> MTDVARLLALRSFTELGARQRARALLDAGSFRELLDPFAGVQSPWLERQGIVPQADDGVVVARGLLDGQPAVLAAIEGAFQGGSLGEVSGAKIAGALELAAEDNRNGVPTRALLLLETGGVRLQEANLGLAAIAEIQAAIVDLQRYQPVVAVIAGPVGCFGGMSIAAGLCSYVLVTREARLGLNGPQVIEQEAGIAEYDSRDRPFIWSLTGGEQRFASGLADAYLADDLDEVRTSVLAYFAKGL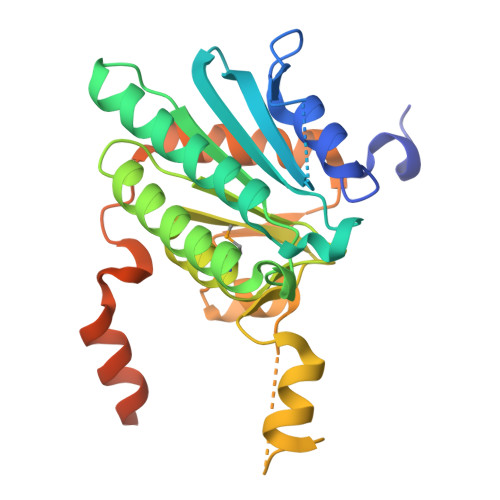PARPRCRRAEDYLRRLGDLDTAEQPDAAGVRRLYQGLGQGDAT> GSHMIDVIIAGGGPTGLMLAGELRLHGVRTVVLEKEPTPNQHSRSRGLHARSIEVMDQRGLL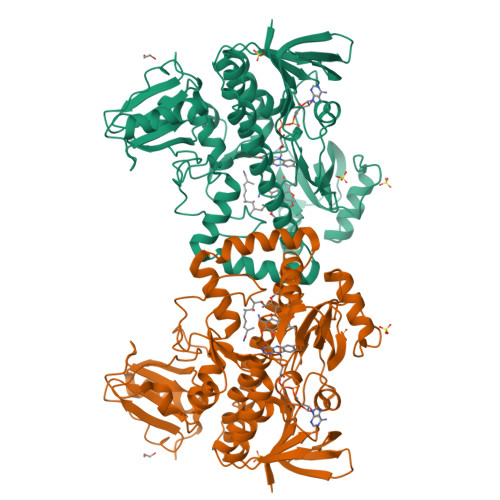ERFLAHGEQFRVGGFFAGLAAEWPADLDTAHSYVLAIPQVVTERLLTEHATELGAEIRRGCEVAGLDQDADGVTAELADGTRLRARYLVGCDGGRSTVRRLLGVDFPGEPTRVETLLADVRIDVPVETLTAVVAEVRKTQLRFGAVPAGDGFFRLIVPAQGLSADRAAPTLDELKRCLHATAGTDFGVHSPRWLSRFGDATRLAERYRTGRVLLAGDAAHIHPPTGGQGLNLGIQDAFNLGWKLAAAIGGWAPPDLLDSYHDERHPVAAEVLDNTRAQMTLLSLDPGPRAVRRLMAELVEFPDVNRHLIEKITAIAVRYDLGDGHDLVGRRLRDIPLTEGRLYERMRGGRGLLLDRTGRLSVSGWSDRVDHLADPGAALDVPAALLRPDGHVAWVGEDQDDLLAHLPRWFGAAT>GSHMNTSRFESLTGSVDVLFPEYDDPPSEPITLLKRWLATADVARVREPKALALATATSDGRISSRVIAFSSIDDRGVIFCTHSTSRKGRELTETGWASGLLYWRETGQQIMISGQAVPLEESENDKLWFGRSVPMHAMSSASHQSDELVDREALRAHAAELLALGVALPRPPR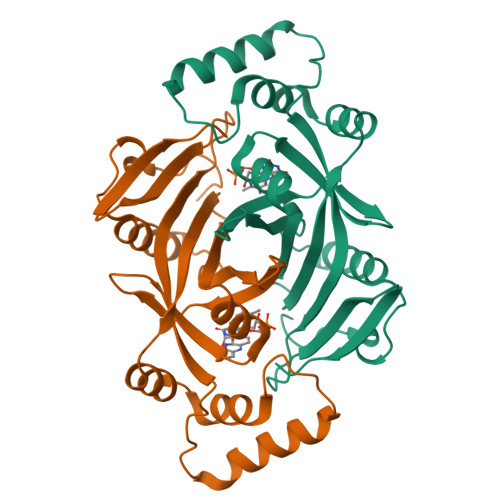FVGYRLEPHEMEFWAASSDRLHRRLRYERDGNDWKTTQLQP[2x]> STAGKVIKCKAAVLWEEKKPFSIEEVEVAPPKAHEVRIKMVATGICRSDDHVVSGTLVTPLPVIAGHEAAGIVESIGEGVTTVRPGDKVIPLWTPQCGKCRVCKHPEGNFCLKNDLSM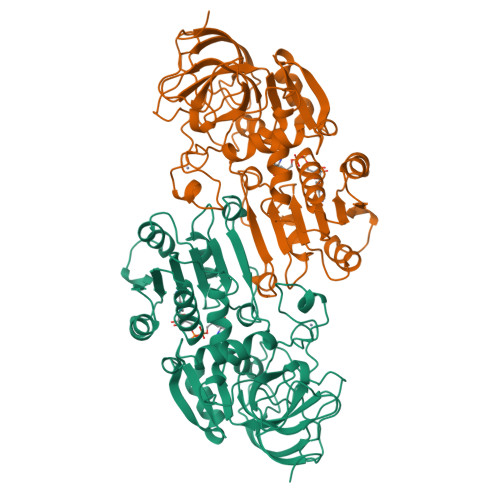PRGTMQDGTSRFTCRGKPIHHFLGTSTFSQYTVVDEISVAKIDAASPLEKVCLIGCGFSTGYGSAVKVAKVTQGSTCAVFGLGGAGLSVIMGCKAAGAARIIGVDINKDKFAKAKEVGATECVNPQDYKKPIQEVLTEMSNGGVDFSFEVIGRLDTMVTALSCCQEAYGVSVIVGVPPDSQNLSMNPMLLLSGRTWKGAIFGGFKSKDSVPKLVADFMAKKFALDPLITHVLPFEKINEGFDLLRSGESIRTILTF>SMRPALYFC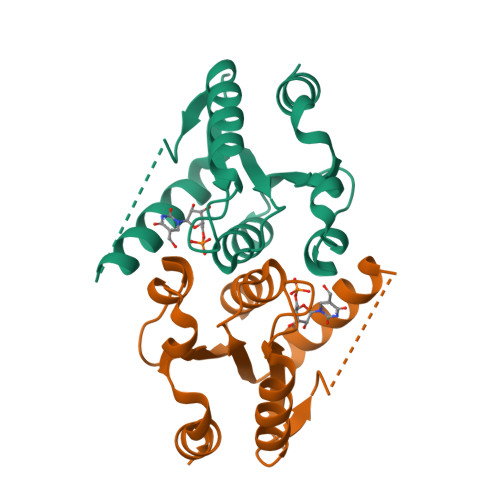GSIRGGREDRTLYERIVSRLRRFGTVLTEHVAAAELGARGEEAAGGDRLIHEQDLEWLQQADVVVAEVTQPSLGVGYELGRAVAFNKRILCLFRPQSGRVLSAMIRGAADGSRFQVWDYEEGEVEALLDRYFEADP[2x]> 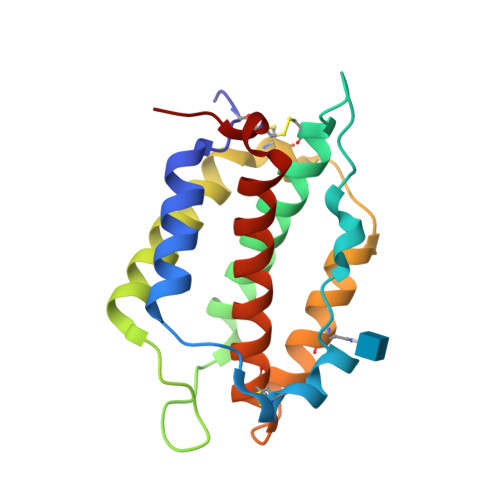PTCQLEGDLVQSAHHLLRDLGADFPEHCLPYNAQISFPSSAFPAATANHPQCHKSLWVVHESLREAGLVFQDNDIPVGEGGVTWNDQKLEDFQNLQYRLVEEGSCLSSVNGSGVLSSYFSNVTAVLQEQDSAACGWMALRRDLLWVLKSALQKHRTCFTWR> MSLAAARGGVGAGPDVRPVHGVHARMAEKMTLSHKEIPTAKASVEVICAELLRLRDRFVSAAPEITPFALTLRLLVIALKHNVILNSTWVDSGEGPQVHVHRGVHLGFGAATERGLLVPVVTDAQDKNTRELASRVAELITGAREGTLTPAEL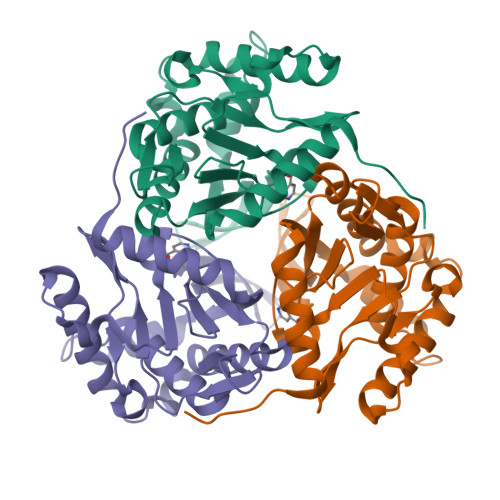RGSTFTVSNFGALGVDDGVPVINHPEAAILGLGAIKPRPVVVGGEVVARPTMTLTCVFDHRVVDGAQVAQFMCELRDLIESPETALLDLEGHHHHHH>[2x]MKDTYTNPVGGITGIGDPYVLKHESRYYLYATSAINRGFKVWESPNLVDWELKGLALDSYY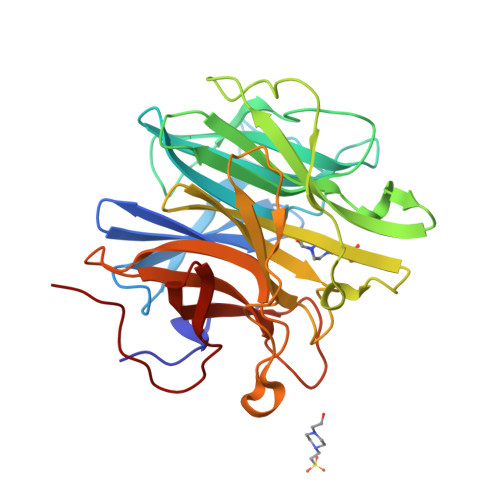EKNGWGTEDFWAPEVIFYNNKFYMTYSARDNDGHLKIALASSKSPLGPFKNIKAPLFDRGLSFIDAHIFIDQDGTPYIYYVKDCSENIINGIHISQIYVQEMSQDLLELKGDPVLAIQPSQDWEGINDAWQWNEGPFVIKHEGKYYMMYSANCYASPDYSIGYAVAETPLGPWIKYSGNPILSKRMDKGISGPGHNSVTVSPDGSELFVVYHTHTYPDSPGGDRTVNIDRLYFEDGILKVKGPTRSPQPGPRSN>[2x]EPLDDYVNTQGASLFSVTKKQLGAGSIEECAAKCEEDEEFTCRAFQYHSKEQQCVIMAENRKSSIIIRMRDVVLFEKKVYLSECKTGNGKNYRGTMSKTKNGITCQKWSSTSPHRPRFSPATHPSEGLEENYCRNPDNDPQGPWCYTTDPEKRYDYCDILECEEECMHCSGENYDGKISKTMSGLECQAWDSQSPHAHGYIPSKFPNKNLKKNYCRNPDRE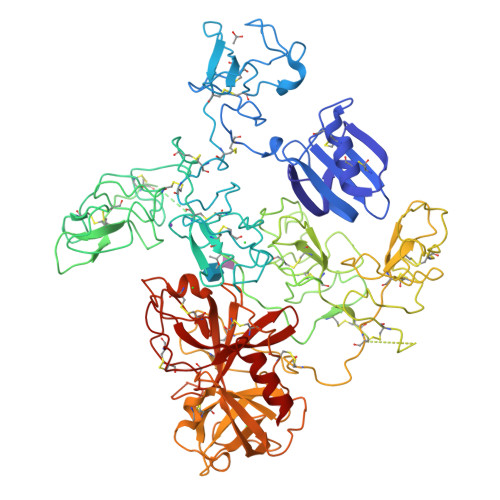LRPWCFTTDPNKRWELCDIPRCTTPPPSSGPTYQCLKGTGENYRGNVAVTVSGHTCQHWSAQTPHTHNRTPENFPCKNLDENYCRNPDGKRAPWCHTTNSQVRWEYCKIPSCDSSPVSTEQLAPTAPPELTPVVQDCYHGDGQSYRGTSSTTTTGKKCQSWSSMTPHRHQKTPENYPNAGLTMNYCRNPDADKGPWCFTTDPSVRWEYCNLKKCSGTEASVVAPPPVVLLPDVETPSEEDCMFGNGKGYRGKRATTVTGTPCQDWAAQEPHRHSIFTPETNPRAGLEKNYCRNPDGDVGGPWCYTTNPRKLYDYCDVPQCAAPSFDCGKPQVEPKKCPGRVVGGCVAHPHSWPWQVSLRTRFGMHFCGGTLISPEWVLTAAHCLEKSPRPSSYKVILGAHQEVNLEPHVQEIEVSRLFLEPTRKDIALLKLSSPAVITDKVIPACLPSPNYVVADRTECFITGWGETQGTFGAGLLKEAQLPVIENKVCNRYEFLNGRVQSTELCAGHLAGGTDSCQGDSGGPLVCFEKDKYILQGVTSWGLGCARPNKPGVYVRVSRFVTWIEGVMRNN>[2x]MTNNPLIPQSKLPQLGTTIFTQMSALAQQHQAINLSQGFPDFDGPRYLQERLA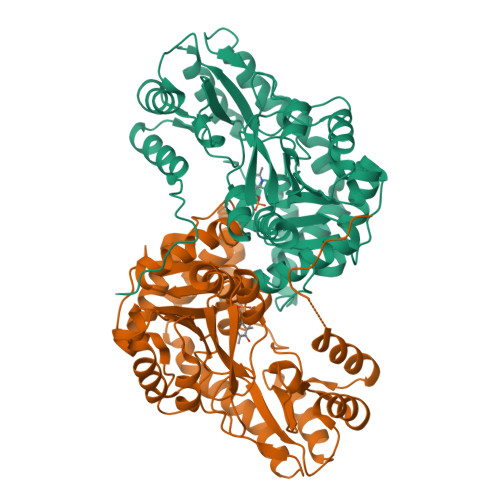HHVAQGANQYAPMTGVQALREAIAQKTERLYGYQPDADSDITVTAGATEALYAAITALVRNGDEVICFDPSYDSYAPAIALSGGIVKRMALQPPHFRVDWQEFAALLSERTRLVILNTPHNPSATVWQQADFAALWQAIAGHEIFVISDEVYEHINFSQQGHASVLAHPQLRERAVAVSSFGKTYHMTGWKVGYCVAPAPISAEIRKVHQYLTFSVNTPAQLALADMLRAEPEHYLALPDFYRQKRDILVNALNESRLEILPCEGTYFLLVDYSAVSTLDDVEFCQWLTQEHGVAAIPLSVFCADPFPHKLIRLCFAKKESTLLAAAERLRQL> GMQKPHLLITSAGRRAKLVEYFVKEFKTGRVSTADCSPLASALYMADQHYIVPKIDEVEYIDHLLTLCQDEGVTALLTLIDPELGLLAQATERFQAIGVTVIVSPYAACELCFDKYTMYEYCLRQGIAHARTYATM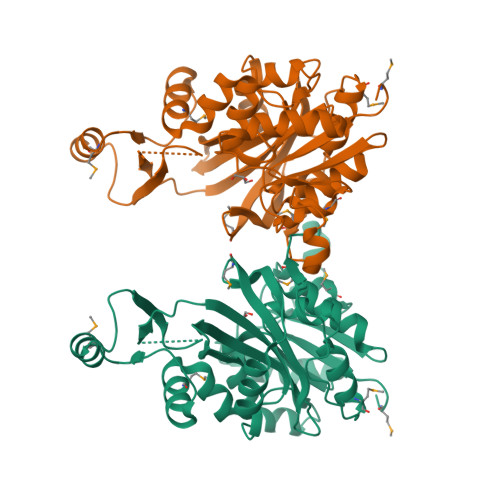ASFEEALAAGEVQLPVFVKPRNGSASIEVRRVETVEEVEQLFSKNTDLIVQELLVGQELGVDAYVDLISGKVTSIFIKEKLTMRAGETDKSRSVLRDDVFELVEHVLDGSGLVGPLDFDLFDVAGTLYLSEINPRFGGGYPHAYECGVNFPAQLYRNLMHEINVPQIGQYLDDIYMLKHDTVTLISAAELQKIKR>ELPDFFQGKHFFLYG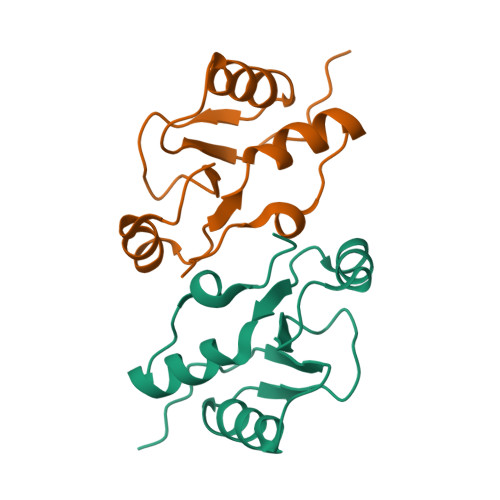EFPGDERRKLIRYVTAFNGELEDYMSDRVQFVITAQEWDPSFEEALMDNPSLAFVRPRWIYSCNEKQKLLPHQLYGVVPQA[2x]> ADPPVVNTAYGRVRGVRRELNNEILGPVVQFLGVPYATPPLGARRFQPPEAPASWPGVRQATTLPPACPQNLHGALPAIMLPVWFTDNLEAAATYVQNQSEDCLYLNLYVPTEDGPLTKKRDEA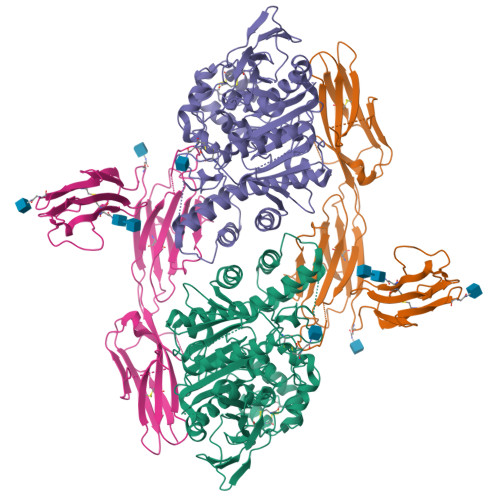TLNPPDTDIRDPGKKPVMLFLHGGSYMEGTGNMFDGSVLAAYGNVIVATLNYRLGVLGFLSTGDQAAKGNYGLLDQIQALRWLSENIAHFGGDPERITIFGSGAGASCVNLLILSHHSEGLFQKAIAQSGTAISSWSVNYQPLKYTRLLAAKVGCDREDSAEAVECLRRKPSRELVDQDVQPARYHIAFGPVVDGDVVPDDPEILMQQGEFLNYDMLIGVNQGEGLKFVEDSAESEDGVSASAFDFTVSNFVDNLYGYPEGKDVLRETIKFMYTDWADRDNGEMRRKTLLALFTDHQWVAPAVATAKLHADYQSPVYFYTFYHHCQAEGRPEWADAAHGDELPYVFGVPMVGATDLFPCNFSKNDVMLSAVVMTYWTNFAKTGDPNQPVPQDTKFIHTKPNRFEEVVWSKFNSKEKQYLHIGLKPRVRDNYRANKVAFWLELVPHLHNLVPR;> ADPQGVYAPAQAQIVHAGQACVVKEDNISERVYTIREGDTLMLQCLVTGHPRPQVRWTKTAGSASDKFQETSVFNETLRIERIARTQGGRYYCKAENGVGVPAIKSIRVDVQYLDEPMLTVHQTVSDVRGNFYQEKTVFLRCTVNSNPPARFIWKRGSDTLSHSQDNGVDIYEPLYTQGETKVLKLKNLRPQDYASYTCQVSVRNVCGIPDKAITFRLTNTTAPPALKLSVNETLVVNPGENVTVQCLLTGGDPLPQLQWSHGPGPLPLGALAQGGTLSIPSVQARDSGYYNCTATNNVGNPAKKTVNLLVRSMKLVPR>SNAMKNKLPPFIEIYRALIATPSISATEEALDQSNADLITLLADWFKDLGFNVEVQPV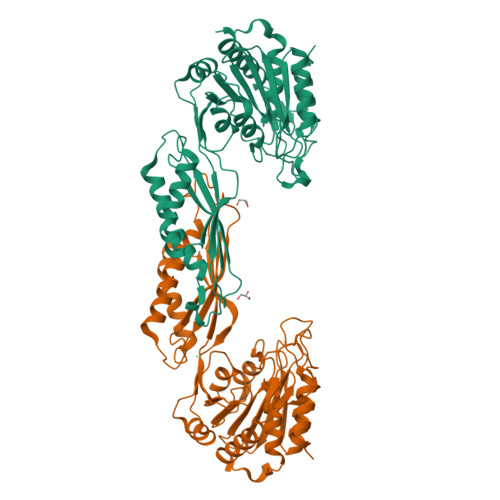PGTRNKFNMLASTGQGAGGLLLAGHTDTVPFDDGRWTRDPFTLTEHDGKLYGLGTADMKGFFAFILDALRDVDVTKLKKPLYILATADEETSMAGARYFAETTALRPDCAIIGEPTSLQPVRAHKGHISNAIRIQGQSGHSSDPARGVNAIELMHDAIGHILQLRDNLKERYHYEAFTVPYPTLNLGHIHGGDASNRICAWCELHMDIRPLPGMTLNELNGLLNDALAPVSERWPGRLTVDELHPPIPGYECPPNHQLVEVVEKLLGAKTEVVNYCTEAPFIQTLCPTLVLGPGSINQAHQPDEYLETRFIKPTRELITQVIHHFCWH[2x]> GPMDELPSLLEVHNVRIVGMG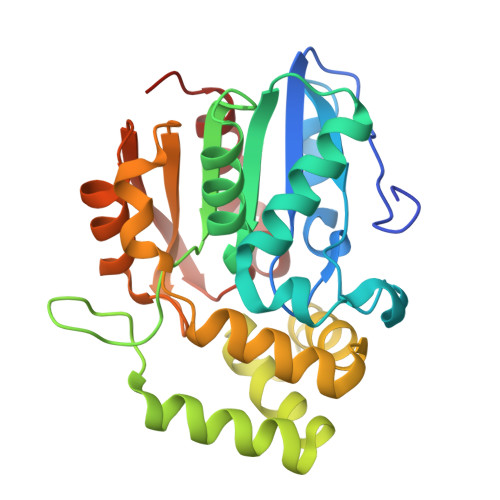EELVVLAHGFGTDQSVWKHVIPHLVDDYRVILFDNMGAGTTDPEYFSFSRYSTLYGYADDLLTILDELEVQSCIFVGHSVSGMVGCLASLYRPEIFSKIITISASPRYLNDMDYFGGFEQEDLNQLFEAMQSNFKAWVSGFAPLAVGADIDSMAVQEFGRTLFNIRPDIAFSVAKTIFQSDLRSILPKVTVPCHILQSSKDLAVPVVVADYLHLTLGGPTIVEVLPTEGHLPQLSSPDIVIPVLKRHVAGNLESC> DYL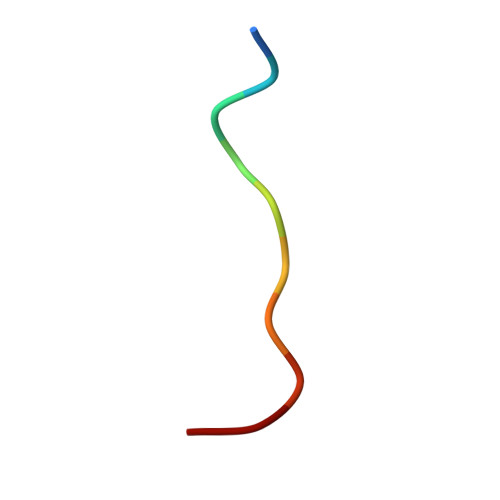DIPAFLR>MTVSRRGFMAGLALTGAAALPVAYYTHRHLTREEEPQTPDEASLDLAATDGIRLGDRLRGLWDLRLVGGDAELPGLPREGLQLVLDVAPKGRGLIGYLDTPERLLAAEPPRFRVLGDLLGASSASIRWRLVDQASGSVAPTHDCSAVFDEVWADYANAGDGTLSGRIQRLERSPLSPNEDFRFVAVKRHFPLAHERIVLNEKLLGWLVSPQHRLFHQLWHASRDKWHRLSEKQRNALRGVGWQPGPLDRERDARGPRKDRNASGIDFFFMHRHMLHTARSMQDLPSWERLPRPVVPLEYDRPGFIRYFDNPDGFSVPPAWVAVDDDEYSEWLHGLKSAEAYHANFLVWESQYQDPAYLAKLTLGQFGSELELGMHDWLHMRWASVTRDPSNGAPVMTDRFPADFAPRWFRPENDFLGDPFSSHVNPVFWSFHGWIDDRIEDWYRAHERFHPGEVQRREVEGIQWFAPGRWVEVGDPWLGPATHGCGLSDVQASSNSVELDVET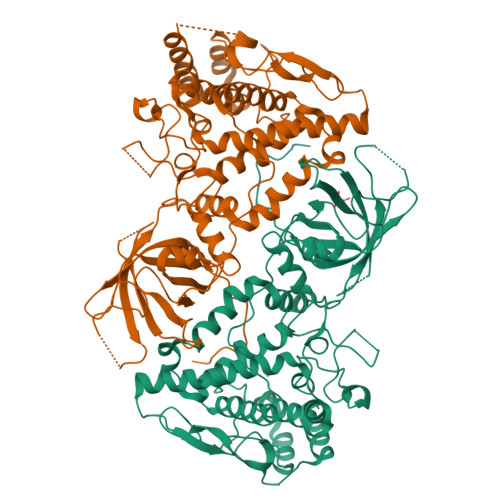MKLALRIIFSEEDQLSGWLKRAPRRPWYARNLKLARDQLRR[2x]> MHHHHHHGYKMVNPPRVVGNWTPKDLSFEYKDVEITTEDNVKLSGWWIDNGSDKTVIPLHGYTSSRWAEHYMRPVIEFLLKEGYNVLAFDFRAHGKSGGKYTTVGDKEILDLKAGVKWLKDNYPEKSKRIGVIGFSMGALVAIRGLSEVKEICCGVADSPPIYLDKTGARGMKYFAKLPEWLYSFVKPFSELFSGGRPINVLNYTNSIKKPLFLIIGRRDTLVKVE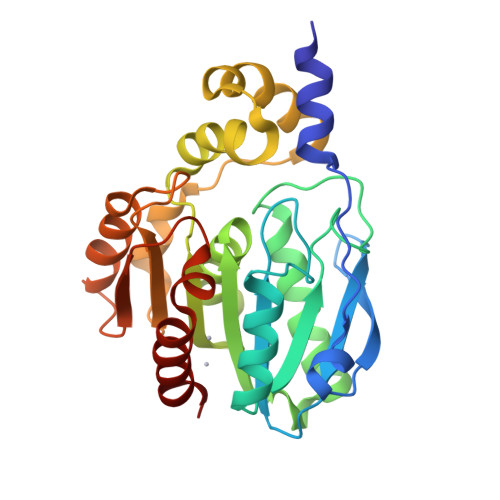EVQEFYERNKHVNPNVELWVTDAPHVRTIQVFPEEWKSRVGEFLKRWMG> MSNTGGNGNDNAAPSLSTTTENVNGNDDTPSSNLTINDLGGSKFPPQPKKSKQQQQQNITDRLSTFSNFFEDEKLDKDDMKLEFDKIEKKLCDIFETDTIPNNASKDQITSGKIKIKGEEITISKEAQDFTLELSSLLNLDQILTFILIREYLTNNNNKVLNYDKSELFNLLDYYYNERASLLCILGSIIKKESSQSKYSSFLKPFIEKNRASIESRLLSYLISFYNFTIPSNLEELQQFYCSSIIKEQLIIVETLFSYNYLKVKKSGNCSNSSSNMNDVNELLIILKKINQLQIGSYSDQLIGILNSMKRNSEVIQWLKRIEYVLVLLVFCNNRDLLRHESLQQNELEIINTITTLSQSIHYNAPLATSLFFTIINLFISTSSSSSSSSPSSSSSVNFSNSLQQYFTKASSQYDPIDYIFNCLSNGFNDSTYLAGYCDCIHIFLNRFSEVISLTDVSEQHVDRIIDIYCMLHEKGGEVLSSILWSERSNDPVYQFSISPDCLNRNPDRVLSILKSIIINDTSSQAVFNELILININNQSSSKQIISFNDFNKVKEVLDITNDDGNGTISGVMKRDIISQSFRLYKSQFKSFSVINDGSGGDGGIEIVFTLHDLIIDLVAIEFNSFLDSLGQQAFFDQRTIEVSKAYIVVLDLISKLVNFTPDSYSKYFWQLFENNRILESIIQVYLRLCNQQNFTVNSIPTNINIKESNGNGGFQQKINKQQQQQPTLMSSYSTAHYNFNIITNVITSILSLFTSFSKMNPLPILNLLIEKGIWSSSPTVLISLFKRGSFNHLYDVEKRSSTTSSTSSTSSSSLSSSTFPLTKSIVKLFNTFINPLNQFEKCIDRSQYIGYLESFISFHLQVISDYPIISGNNNHNETWEMISEIFSALDFILNKSQSRNSILKSLAFKIICSFSGGILQCTLSSLLDLEVLQNTNKSIDRTSSIDNILKSSLKFSKSILSTIYLSIVLKRSNKINNNNQNNDNNNENNNNNNNGDNNNNNNNNENNNNNENNDNINDNNIENYENEYSNNLVEQFLTTFFIVKQNETNLLIDQEDRNGLTSTIVTNSITTETITSKTDYNNLFIVLFNYINIISDCQDIQILSCEILSSLVRILRVLESNFSVSTLFNTDEPFILMIEKFSKKFIINNNEFDVWSLQLKTNILRLLVESSTNQIYFINRLLNCENNNINNNNNNNDDSGGDKKNKSFIIKLLLDRNVSINDNSEFSLALFQLVNNLYCNSIYYDSFVDQLNNTQDFWNLLLDMQKTINEEEEQEEESIINEELIC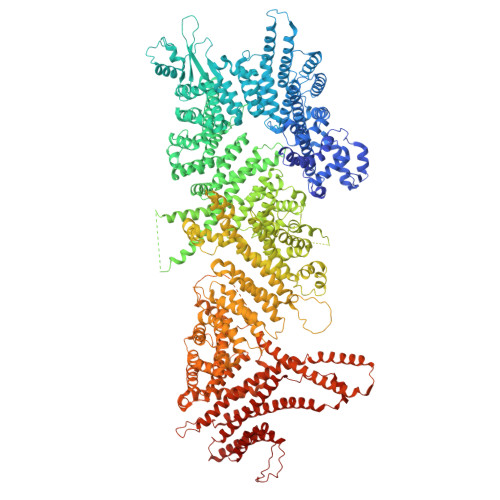KKLKITYAIEILSLSVLLSSDITTATTTVGNLVCSTLSNNKWNEIFKNNKSGIVNMINNYYFQFIDLENVFPIQKIRDYWMVNNLPSPDQLQTTIAYQYFPNINNNIPIVELFAIDTIIETSKQFNDQYYLELLIQRNLFELLTTTNLCLSRAFSKLFRVILMKQPQNFININGGSGSGSGSSNSGVPLSTILHTLVDKATSIENQSIKTLVVRNDILMFLCESISTASHLWCKSCPIESVDIEILSKLSNLLAQCSSNPILGHSISYHILTSILILVENTSQHQYIEIKVFNQLINTLSLFITEPHFRVPPISSMDGTTTTTTSGGNVGEGKTINGKQKKPLPSICNLSIYLLQVLIDRLDPNALIAAFPNNLLENLAKLLKNSLNMVNGNQIDNITASSVLNLLISFCKQPLVSEQLLDNRIIQLLSDHSLKYLQFSMDPYLASTEISAATASIYGGINYYFHNNDDDYDNHRQFNQKKNKWHRVWTLVIKFLISVSKPLESSERFIEQLSNFILSHKDRLFYYFDLFNEFGATQHSQYFTKQWFQQLEYITSLFSIFTKYTKRYYLSMNIYREFLSLAYRLLVSISIQCSELNFIENNFIPITKNEKHKNLVQVKEFIDDSQRLQQQQLQQQQQLQQSQLQQSTPYRTSHYQQQLLQLQQQLQKQQQPQQQNIQNSFFKFSIESNYTHIINNCFTILIRINEYVRSSNEFVPQLTIYPNVATFGTFGQLSQYIISKLFQISNVVDKLSRNNNNNNNNNNNNNSSSIYNNLEDQNSISVDELLDLNLYKTKIKQTLEKNTLLLILYAKQTPPSTSPQETLRENQVNNIITHLLKQQFNNNNNNNNFSQNRTPLKNNNNNLNNNNTSENDENDEFLNFLSDLQRVK> MGSSHHHHHHSSGHMFKYEDIPA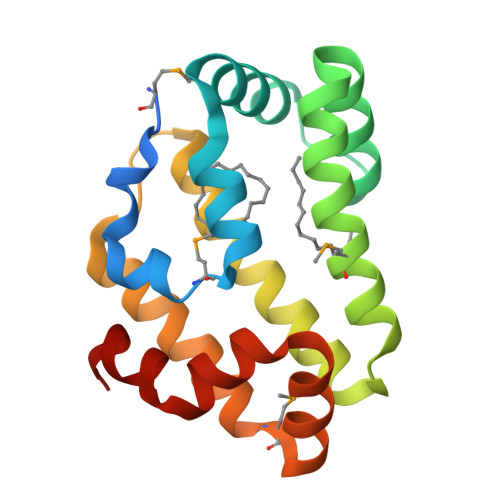DYRDLMPPEARDFLQNLSDGDKTVLKEVFKAGPYKNTEESIAALKKKSPELGAKVEKLHAMVKSKIAALGPEAKGFAEKSIEIARGIKARYYTGNEPTKDDLKASVKEVLKLYKAMSDAGKADFGKQFPFLAKVFESGKAAKFAGEN DENDRON-D1 | C31 H50 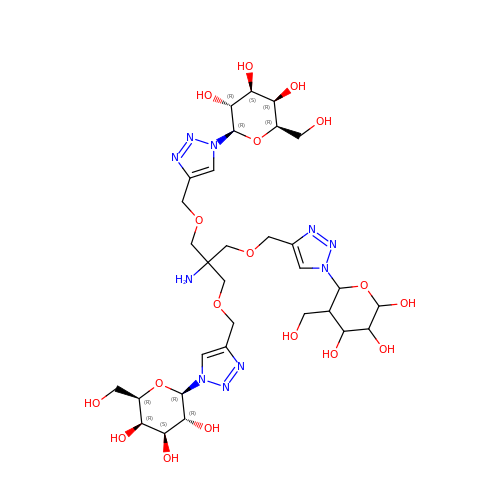N10 O18 | VLZLQHDSQRKRHA-NBVMFUKPSA-N>[4x]MHGSNKLPGFATRAIHHGYDPQDHGGALVPPVYQTATFTFPTVEYGAACFAGEQAGHFYSRISNPTLNLLEARMASLEGGEAGLALASGMGAITSTLWTLLRPGDEVLLGN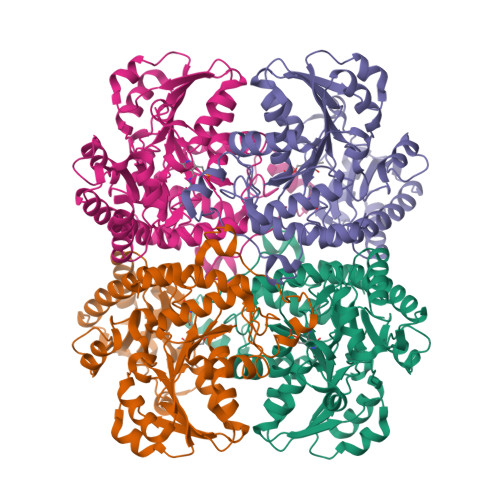TLYGCTFAFLHHGIGEFGVKLRHVDMADLQALEAAMTPATRVIYFESPANPNMHMADIAGVAKIARKHGATVVVDNTYCTPYLQRPLELGADLVVHSATKYLSGHGDITAGIVVGSQALVDRIRLQGLKDMTGAVLSPHDAALLMRGIKTLNLRMDRHCANAQVLAEFLARQPQVELIHYPGLASFPQYTLARQQMSQPGGMIAFELKGGIGAGRRFMNALQLFSRAVSLGDAESLAQHPASMTHSSYTPEERAHYGISEGLVRLSVGLEDIDDLLADVQQALKASA2,5-DITERT-BUTYLBENZENE-1,4-DIOL | 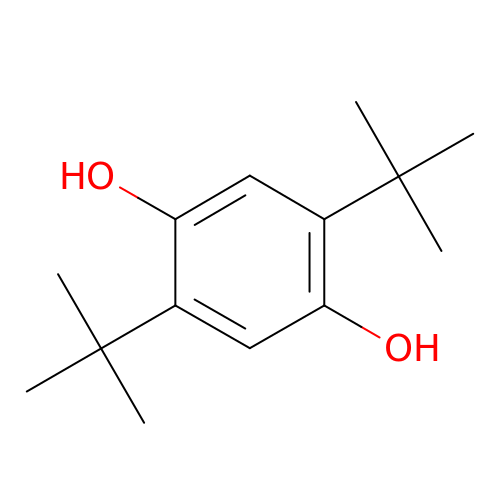C14 H22 O2 | JZODKRWQWUWGCD-UHFFFAOYSA-N>MPMTLGYWNIRGLAHSIRLLLEYTDSSYEEKKYTMGDAPDYDRSQWLNEKFKLGLDFPNLPYLIDGTHKITQSNAILRYIARKHNLCGESEKEQIREDILENQFMDSRMQLAKLCYDPDFEKLKPEYLQALPEMLKLYSQFLGKQPWFLGDKITFVDFIAYDVLERNQVFEPSCLDAFPNLKDFISRFEGLEKISAYMKSSRF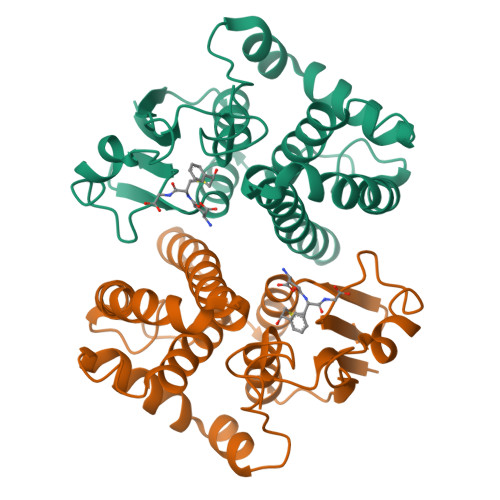LPRPVFSKMAVWGNK[4x]> MSVVPPNRSQTGWPRGVTQFGNKYIQQTKPLTLERTINLYPLTNYTFG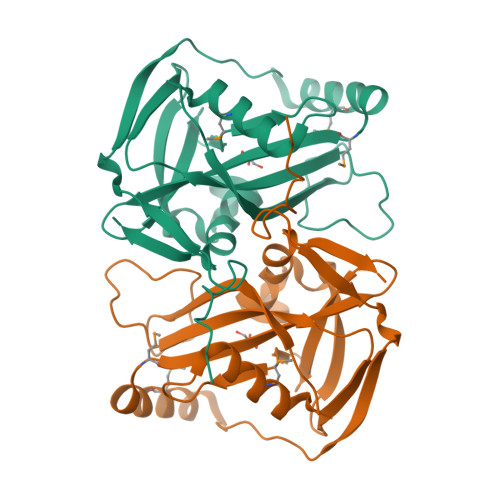TKEPLYEKDSSVAARFQRMREEFDKIGMRRTVEGVLIVHEHRLPHVLLLQLGTTFFKLPGGELNPGEDEVEGLKRLMTEILGRQDGVLQDWVIDDCIGNWWRPNFEPPQYPYIPAHITKPKEHKKLFLVQLQEKALFAVPKNYKLVAAPLFELYDNAPGYGPIISSLPQLLSRFNFIYN>AYSNTYQEFTNIDQAKAWGNAQYKKYGLSKSEKEAIVSYTKSASEINGKLRQNKGVINGFPSNLIKQVELLDKSFNKMKTPENIMLFRGDDPAYLGTEFQNTLLNSNGTINKTAFEKAKAKFLNKDRLEYGYISTSCMNVSQFAGRPIITKFKVAKGSKAGYIDPISAFAGQLEMLLPRHSTYHIDDMRLSSDGKQIIITATMMGTAINPK[4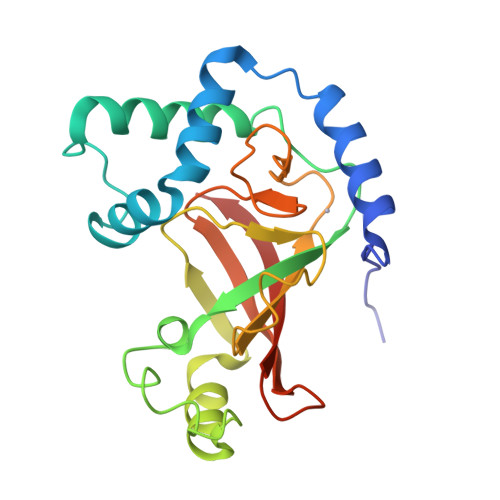x]> MASWDSPTASSNGDLIEEIQASSTSTDPRTFTGLSIVEDIGDVVPVTDNASPALPVSLTDADGNDVVVEDVSRILPLDLYGTYSKTIAGLGLVDNIVGRTVSSTEPALADTEVVTTGGHTLNAEAILNLHPTLVIIDHSIGPREVIDQIRAAGVATVIMSPQRSIASIGDDIRDIASVVGLPEEGEKLAERSVAEVEEASTVVDELTPEDPLKMVFLYAAGTGGVFFILGDAYGGRDLIEGLGGVDMAAEKGIM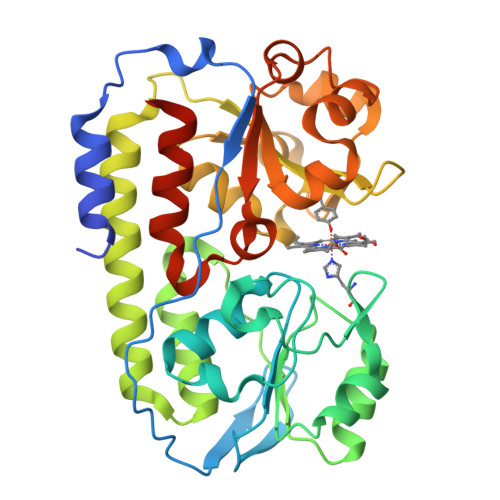DLAPANAEALAELNPDVFVMMSEGLVSTGGIDGLMERPGIAQTTAGQNQRVLALPDGQSLAFGAQTGELLLRASRELYVQGGELEHHHHHH> MDAPMEDAPAPVAQVKVIFTTTEPDLELPESKRQLLVPADIRRYGLSRILNSESMLDTGSIPFDFLINGSFLRSSLEDYLTSNGLSLETTLTLQYVRSLIPPVYEASFEHDDWVSAVDVLSATSPAGRWSSAANSSAAVQPGQERVLSASYDGLLRIWNASGSVIATSPSGSHGGHTASIKAAKFLTSDRLASAGMDRTVRVWKYTESDHFTGELKPTLELYGHTGSVDWLDVDGHSKHILTASADGAIGFWSASKASAPEPDASLLPGAHVSKRRKATSSVSTAQRGPLGLWSIHTAPATAAIFDPRDRTVAYSASQDHTVRTLDLTTGQVVSTLTLTHPLLSLSALTRAGTTSPLLAAGTSARHITMVDPRASSATTSVMTLRGHANKVVSLSPSPENEYSLVSGSHDGTCRVWDLRSVRPATKEEGSLGGVSEPVYVIERESWASKGKKKRPVAGDGCKVFSVVWDKLGIFSGGEDKKVQVNRGRNIVTEQK;> MAHHHHHHSAALEVLFQGPGPSPDELKPFPTVQQTIFRGHEGRVRSVAIDPTGVALATGGDDGTVRVWELLTGEQVWSVKLNGDEAVNTVRWRPTKDTFILAAAAGEDIFLMIPTHPSVTPALDQASRDILNAGFGHATNGKQQANLPPGKEPPGKWARPGTRLEDEGVLLRITVRSTIKAISWHRRGDHFATVSPSGQRSSVAIHTLSKHLTQIPFRKLNGLAQTASFHPLRPLFFVATQRSIRCYDLQKLELVKIVQPGAKWISSFDVHPGGDNLVVGSYDKRLLWHDLDLSNRPYKTMRFHTEAIRAVRFHKGGLPLFADASDDGSLQIFHGKVPNDQLENPTIVPVKMLKGHKVVNKLGVLDIDWHPREPWCVSAGADG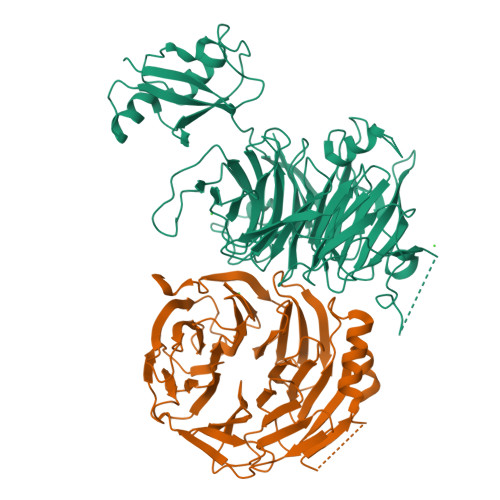TARLWM> SSQIRQNYSTEVEAAVNRLVNLYLRASYTYLSLGFYFDRDDVALEGVCHFFRELAEEKREGAERLLKMQNQRGGRALFQDLQKPSQ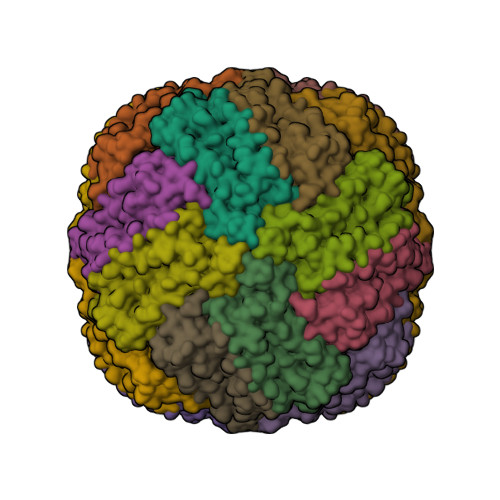DEWGTTPDAMKAAIVLEKSLNQALLDLHALGSAQADPHLCDFLESHFLDEEVKLIKKMGDHLTNIQRLVGSQAGLGEYLFERLTLKHD> IKNASIKRKL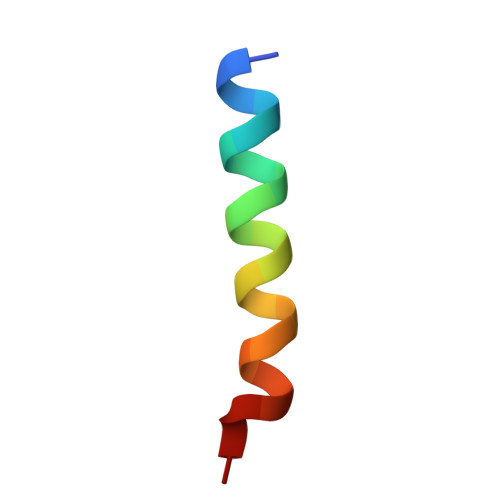FGLANTIREQAL> MACAAARSPADQDRFICIYPAYLNNKKTIAEGRRIPISKAVENPTATEIQDVCSAVGLNVFLEKNKMYSR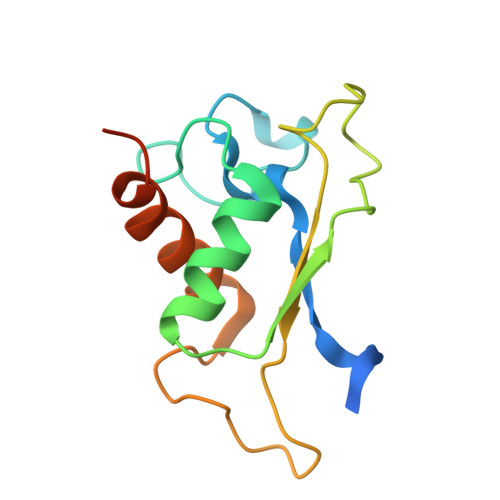EWNRDVQYRGRVRVQLKQEDGSLCLVQFPSRKSVMLYAAEMIPKLKTRTQLEHHHHHH> MAAPVVAPPGVVVSRANKRSGAGPGGSGGGGARGAEEEPPPPLQAVLVADSFDRRFFPIS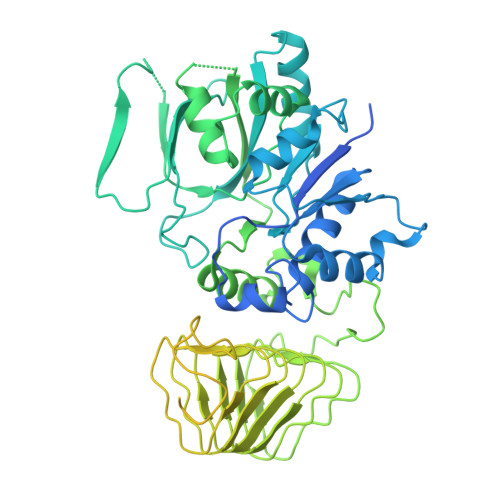KDQPRVLLPLANVALIDYTLEFLTATGVQETFVFCCWKAAQIKEHLLKSKWCRPTSLNVVRIITSELYRSLGDVLRDVDAKALVRSDFLLVYGDVISNINITRALEEHRLRRKLEKNVSVMTMIFKESSPSHPTRCHEDNVVVAVDSTTNRVLHFQKTQGLRRFAFPLSLFQGSSDGVEVRYDLLDCHISICSPQVAQLFTDNFDYQTRDDFVRGLLVNEEILGNQIHMHVTAKEYGARVSNLHMYSAVCADVIRRWVYPLTPEANFTDSTTQSCTHSRHNIYRGPEVSLGHGSILEENVLLGSGTVIGSNCFITNSVIGPGCHIGDNVVLDQTYLWQGVRVAAGAQIHQSLLCDNAEVKERVTLKPRSVLTSQVVVGPNITLPEGSVISLHPPDAEEDEDDGEFSDDSGADQEKDKVKMKGYNPAEVGAAGKGYLWKAAGMNMEEEEELQQNLWGLKINMEEESESESEQSMDSEEPDSRGGSPQMDDIKVFQNEVLGTLQRGKEENISCDNLVLEINSLKYAYNISLKEVMQVLSHVVLEFPLQQMDSPLDSSRYCALLLPLLKAWSPVFRNYIKRAADHLEALAAIEDFFLEHEALGISMAKVLMAFYQLEILAEETILSWFSQRDTTDKGQQLRKNQQLQRFIQWLKEAEEESSEDD>[4x]KKIVEVKHPLVKHKLGLMREQDISTKRFR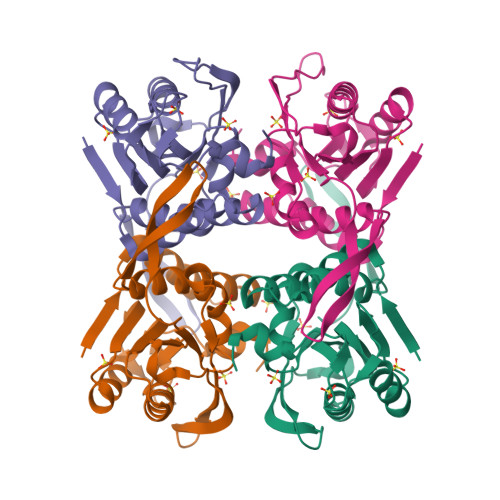ELASEVGSLLTYEATADLETEKVTIEGWNGPVEIDQIKGKKITVVPILRAGLGMMDGVLENVPSARISVVGMYRNEETLEPVPYFQKLVSNIDERMALIVDPMLATGGSVIATIDLLKKAGCSSIKVLVLVAAPEGIAALEKAHPDVELYTASIDQGLNEHGYIIPGLGDAGDKIFGTK> KVQTDPPSVPICDLYPNGVFPKGQECEYPPTQDGRTAAWRTTSEEKKALDQASEEIWNDFREAAEAHRQVRKYVMSWIKPGMTMIEICEKLEDCSRKLIKENGLNAGLAFPTGCSLNNCAAHYTPNAGDTTVLQYDDICKIDFGTHISGRIIDCAFTVTFNPKYDTLLKAVKDATNTGIKCAGIDVRLCDVGEAIQEVMESYEVEIDGKTYQVKPIRNLNGHSIGQYRIHAGKTVPIIKGGEATRMEEGEVYAIETFGSTGKGVVHDDMECSHYMKNFDVGHVPIRLPRTKHLLNVINENFGTLAFCRRWLDRLGESKYLMALKNLCDLGIVDPYPPLCDIKGSYTAQFEHTILLRPTCKEVV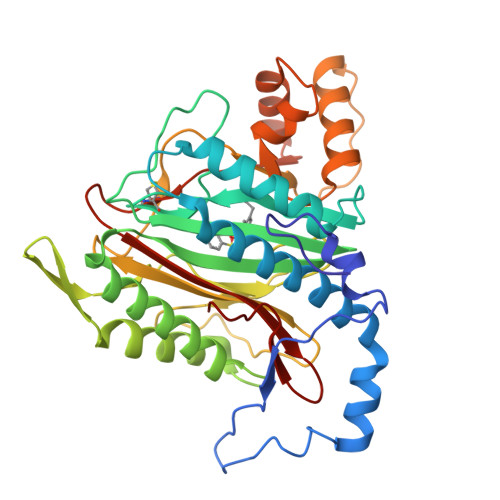SRGDDY> CPERELQRREEEANVVLTGTVEEIMNVDPVHHTYSCKVRVWRYLKGKDIVTHEILLDGGNKVVIGGFGDPLICDNQVSTGDT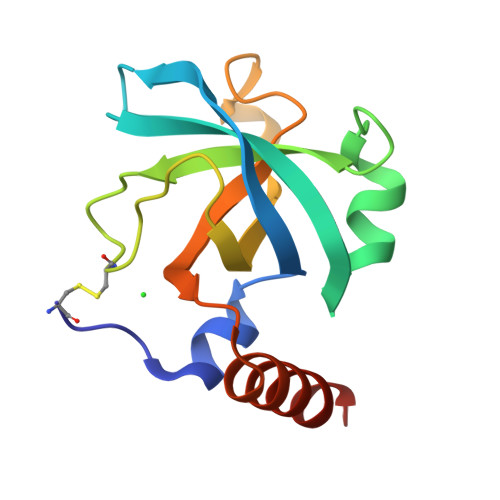RIFFVNPAPQYMWPAHRNELMLNSSLMRITLRNLEEVEHCVEEHRKLKA>[2x]MLNQELELSLNMAFARAREHRHEFMTVEHLLLALLSNPSAREALEACSVDLVALRQELEAFIEQTTPVLPASEEERDTQPTLSFQRVLQRAVFHVQSSGRNEVTGANVLVAIFSEQESQAAYLLRKHEVSRLDVVNFISHGTR;>[2x]MGKTNDWLDFDQLAEEKVRDALKPPSMYKVILVN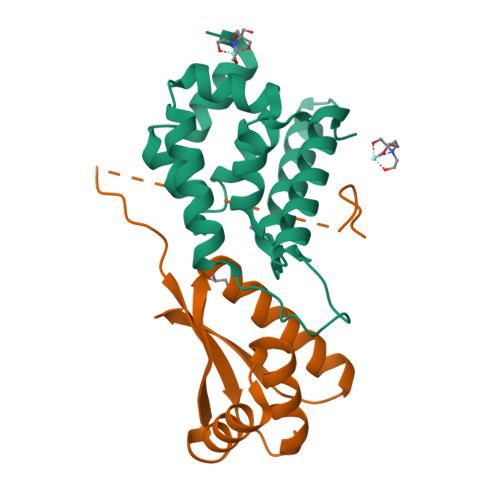DDYTPMEFVIDVLQKFFSYDVERATQLMLAVHYQGKAICGVFTAEVAETKVAMVNKYARENEHPLLCTLEKA>[2x]SAMMYIQELRSGLRDMHLLSCLESLRVSLNNNPVSWVQTFGAEGLASLLDILKRLHDEKEETSGNYDSRNQHEIIRCLKAFMNNKFGIKTMLETEEGILLLVRAMDPAVPNMMIDAAKLLSALCILPQPED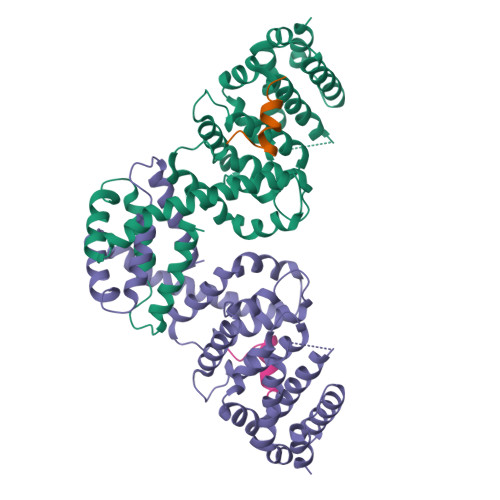MNERVLEAMTERAEMDEVERFQPLLDGLKSGTSIALKVGCLQLINALITPAEELDFRVHIRSELMRLGLHQVLQELREIENEDMKVQLCVFDEQGDEDFFDLKGRLDDIRMEMDDFGEVFQIILNTVKDSKAEPHFLSILQHLLLVRNDYEARPQYYKLIEECVSQIVLHKNGTDPDFKCRHLQID;>[2x]MRRAKLAKEKAEKERLEKQQKREQLIDMNAEGDETGVMDSLLEALQSGAAFRRKRG In this study, we apply a novel rational design approach to the stabilization of wild-type Amadoriase I from Aspergillus fumigatus. Using a rational in silico computational design and screening method, we have produced two forms of the deglycating enzyme Amadoriase I featuring a significantly higher thermostability compared to the WT enzyme. In particular, the introduction of disulfide bonds provide considerable stability to proteins by locking their fold in a well-defined local or global conformation. We used X-ray crystallography to confirm the introduction of the designed disulfide bonds in the mutant enzymes.

To confirm the formation of the designed disulfide bond in the SS03 and in the SS17 mutants and to assess any possible change that such modifications may have caused to their global molecular architecture relative to the wild-type enzyme, we solved the crystal structures of these two thermostabilized species. The crystal structures of the SS03 and the SS17 mutants were determined at 2.15 and 2.85 Å resolution, respectively. The overall fold of the two mutants is very similar to that of the wild-type enzyme, with an RMSD for main chain atoms of 0.268 and 0.804 Å for SS03 and SS17, respectively. Focusing on the region where the mutations were introduced, the SS03 mutant (S67C/P121C) is highly superimposable to the wild type enzyme (residues 62 to 72 and 116 to 126, RMSD = 0.842) while the SS17 variant (D295C/K303C) shows a structural rearrangement in the region from residue 290 to 308, with an RMSD of 1.657 Å. No significant variation in the geometry of the catalytic pocket can be observed between the two mutants and the wild type enzyme, demonstrating that indeed the introduction of these disulfide bonds, which is intended for thermal stabilization only, does not alter the architecture of the active site of the enzyme. For the SS03 and the SS17 species, the mutations did not significantly affect the apparent steady state parameters relative to the WT. Conversely, the SS03 mutant features a ~3 °C higher thermostability with respect to the WT. On the other hand, the SS07 is more stable in a reducing environment, further confirming the detrimental effect of the introduced disulfide bond in this species. Interestingly, the SSDM, which potentially carries both disulfide bonds of SS03 and SS17 does not display any cooperative effect relatively to the two single mutants; in fact, the measured T50 is consistent with the one obtained for the SS03 mutant, suggesting that only the C67-C121 disulfide bond may be actually formed.

>[2x]HHHHHHSSGHIDDDDKMAPSILSTESSIIVIGAGTWGCSTALHLARRGYKDVTVLDPHPVPSPIAAGNDINKIMEHSELKDGCSDPRSAAFSTFTRAALKAWKTDPVFQPYFHETGFIISGHTPALIDHIRKDEVECSETNFVKLETAEDFRRTMPPGVLTGDFPGWKGWLHKSGAGWIHAKKAMISAFNEAKRLGVRFVTGSPEGNVVSLVYEDGDVVGARTADGRVHKAHRTILSAGAGSDSLLDFKKQLRPTAWTLCHIQMGPEEVKQYRNLPVLFNIAKGFFMEPDEDKHELKICDEHPGYCNFLPDPNRPGQEKSVPFAKHQIPLEAEARARDFLHDTMPHLADRPLSFARICWDADTPDRAFLIDRHPEHPSLLVAVGGSGNGAMQMPTIGGFIADALESKLQKEVKDIVRWRPETAVDRDWRATQNRFGGPDRIMDFQQVGEDQWTKIGESRGP3-(AMINOCARBONYL)-1-[(3R,4S,5R)-3,4-DIHYDROXY-5-METHYLTETRAHYDRO-2-FURANYL]PYRIDINIUM | C11 H18 N2 O4 | 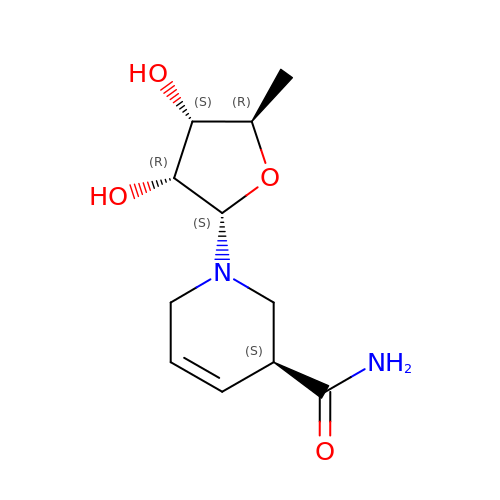MYKCTORFOIHUSG-LALMQGGXSA-N>MASITDKDHQKVILVGDGAVGSSYAYAMVLQGI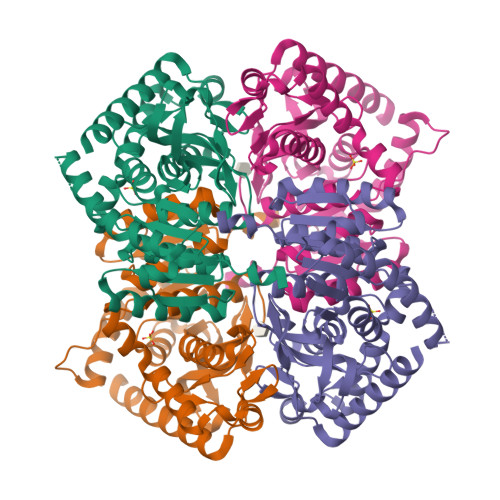AQEIGIVDIFKDKTKGDAIDLSNALPFTSPKKIYSAEYSDAKDADLVVITAGAPQKPGETRLDLVNKNLKILKSIVDPIVDSGFNGIFLVAANPVDILTYATWKLSGFPKNRVVGSGTSLDTARFRQSIAEMVNVDARSVHAYIMGEHGDTEFPVWSHANIGGVTIAEWVKAHPEIKEDKLVKMFEDVRDAAYEIIKLKGATFYGIATALARISKAILNDENAVLPLSVYMDGQYGLNDIYIGTPAVINRNGIQNILEIPLTDHEEESMQKSASQLKKVLTDAFAKNDIETRQ[6x]>SDQINQAGITESDGLGEEIEAKAKKILEDYDKQLQHLKKQVEEAKK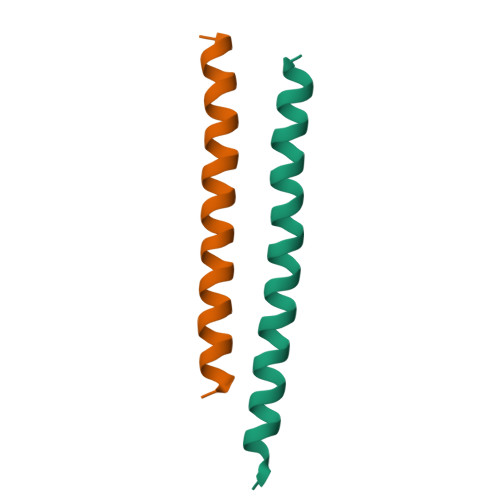DFEEWEKQ[4x]> GSHMDPSPNEIGTVWRDAL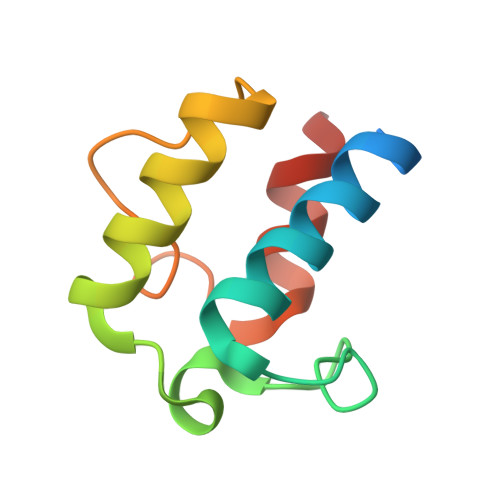KILSEESGLTDEELTDDTSFADVGVDSLMSLVITSRLRDELDIDFPDRALFEECQTIFDLRKRFSGSTE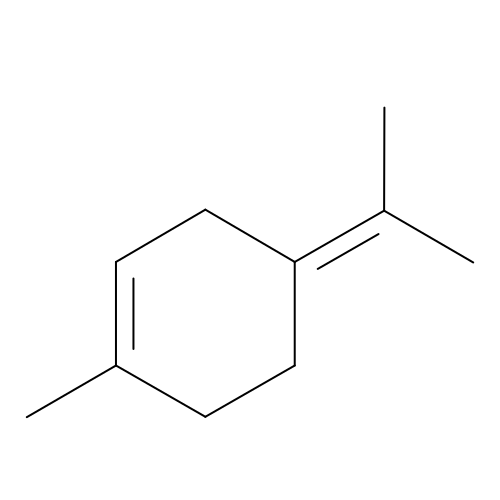1-methyl-4-(propan-2-ylidene)cyclohex-1-ene | C10 H16 | MOYAFQVGZZPNRA-UHFFFAOYSA-N>[2x]MNTRNPDKVVIVGGGTAGWMTASYLKKAFGERVSVTLVESGTIGTVGVGEATFSDIRHFFEFLDLREEEWMPACNATYKLAVRFQDWQRPGHHFYHPFEQMRSVDGFPLTDWWLQNGPTDRFDRDCFVMASLCDAGRSPRYLNGSLLQQEFDERAEEPAGLTMSEHQGKTQFPYAYHFEAALLAEFLSGYSKDRGVKHVVDEVLEVKLDDRGWISHVVTKEHGDIGGDLFVDCTGFRGVLLNQALGVPFVSYQDTLPNDSAVALQVPLDMEARGIPPYTRATAKEAGWIWTIPLIGRIGTGYVYAKDYCSPEEAERTLREFVGPEAADVEANHIRMRIGRSEQSWKNNCVAIGLSSGFVEPLESTGIFFIHHAIEQLVKHFPAGDWHPQLRAGYNSAVANVMDGVREFLVLHYLGAARNDTRYWKDTKTRAVPDALAERIERWKVQLPDSENVFPYYHGLPPYSYMAILLGTGAIGLRPSPALALADPAAAEKEFTAIRDRARFLVDTLPSQYEYFAAMGQRV

Flavin‐dependent halogenases are potentially useful biocatalysts for the regioselective halogenation of aromatic compounds. However, there are a number of flavin‐dependent tryptophan halogenases that can regioselectively halogenate free tryptophan, and therefore have more potential for synthetic purposes. Previously, X‐ray structures have been elucidated for the tryptophan 7‐halogenases, PrnA9 and RebH,10 as well as a tryptophan 5‐halogenase PyrH.11 These structures provided insights into the mechanism and regiocontrol of flavin‐dependent halogenases. It is suggested, that the halogenases utilise O2 to oxidise FADH2 giving C4a‐hydroperoxyflavin, which then reacts with chloride to produce HOCl.

From this, we found that SttH from Streptomyces toxytricini gave good expression in Escherichia coli and catalysed the halogenation of tryptophan to give exclusively 6‐chlorotryptophan. The X‐ray structure of SttH was then determined at 2.7 Å to reveal a dimer, with each monomer exhibiting a box and triangular pyramid structure, as previously observed with PrnA, RebH and PyrH. Within the box structure are the conserved flavin‐dependent tryptophan halogenase sequences GxGxxG and WxWxIP. At the interface with the triangular pyramid, are the catalytic residues K79 and E363, which align with the active‐site lysine and glutamate of PrnA and PyrH. In addition, SttH residues H96 and F98 are positioned for π‐stacking with the indole moiety of the substrate, whilst the P97 carbonyl and Y463 hydroxy groups can potentially hydrogen bond with the indole NH. From sequence alignments it is evident that SttH is more like PyrH than PrnA, with insertions present in PyrH and SttH between residues SttH 155 and 167 and a deletion between SttH 457 and 464 compared with PrnA. Other than residues between SttH G148 and G167, which lack electron density in the SttH structure, the only differences evident in the active‐site region between the structures of PyrH and SttH are those of PyrH residues F451, E452 and T453 and SttH L460, P461 and P462. These residues are of particular interest because they are in close proximity to the active site in PyrH and SttH, and are positioned directly above the α‐amino acid moiety of the substrate, tryptophan. Each of these residues was mutated in SttH to the corresponding residue in PyrH, that is, L460F, P461E and P462T. Interestingly however, the triple mutant SttH L460F/P461E/P462T exhibited similar activity to the wild‐type SttH, with tryptophan as a substrate, but produced 32 % 5‐chlorotryptophan (1 b) and 68 % 6‐chlorotryptophan, whereas the wild‐type SttH only produces the 6‐chlorinated product.>[3x]MMKKIDVKILDPRVGKEFPLPTYATS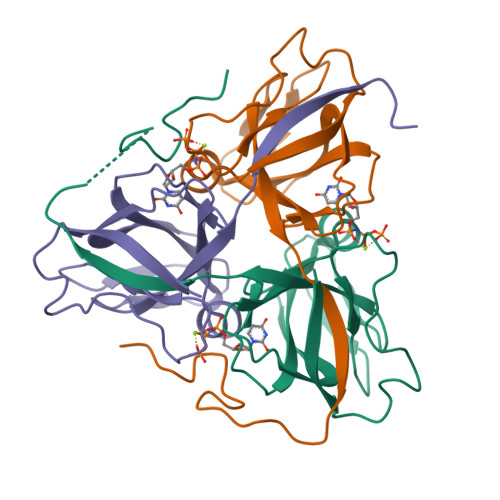GSAGLDLRACLNDAVELAPGDTTLVPTGLAIHIADPSLAAMMLPRSGLGHKHGIVLGNLVGLIDSDYHGQLMISVWNRGQDSFTIQPGERIAQMIFVPVVQAEFNLVEDFDATDRGEGGFGHSGRQ> GPLHMKAVVPGPA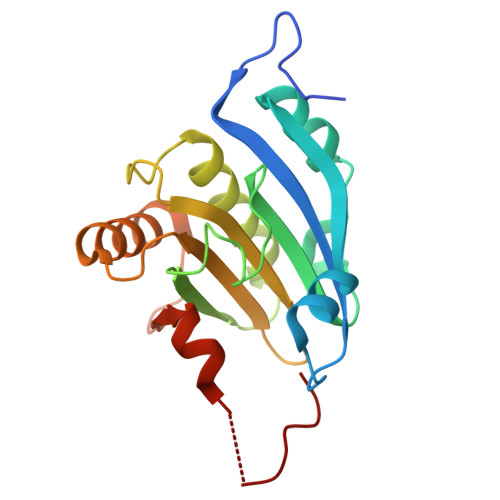EHPLQYNYTFWYSRRTPGRPTSSQSYEQNIKQIGTFASVEQFWRFYSHMVRPGDLTGHSDFHLFKEGIKPMWEDDANKNGGKWIIRLRKGLASRCWENLILAMLGEQFMVGEEICGAVVSVRFQEDIISIWNKTASDQATTARIRDTLRRVLNLPPNTIMEYKTHTDSIKMPGRLGPQRLLF> 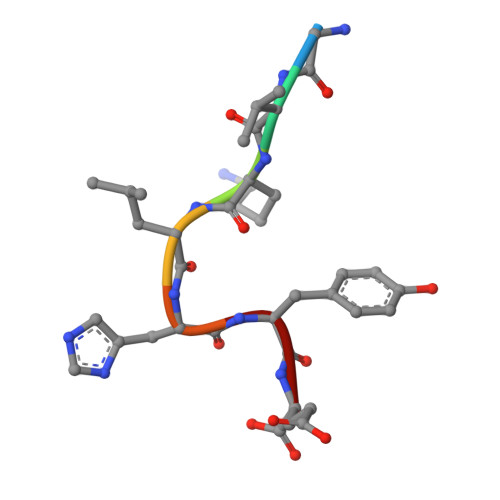GVKLHYE Rhodopsins are seven-transmembrane proteins that contain retinal as a light-absorbing chromophore and a light-induced trans–cis isomerization of retinal triggers their activities. There are, however, 9 genomes from a high salinity environment, 8 were from the same site and showed little genetic variation. Phylogenetic analysis of the amino acid sequences of the rhodopsins encoded by the 56 identified genes revealed that the proteins belonged to four known rhodopsin clades: XLR (3 genes), NaR (1 gene), XeR (15 genes), and CyHR (24 genes) and one novel clade (13 genes); the novel rhodopsin clade consisted entirely of rhodopsin genes from cyanobacterial genomes so we named the clade “cyanorhodopsin” (CyR). All of the CyRs included Lys204N2098R in the seventh helix (helix G), which is known to make a Schiff base linkage between the rhodopsin protein moiety and the retinal chromophore in other rhodopsins. Heterologous rhodopsin gene expression analysis showed that the rhodopsins in the CyR clade function as light-driven outward H+ pumps.

The crystal structures of cell-free-synthesized N2098R and N4075R were determined at 2.65 Å and 1.9 Å resolution, respectively. The N2098R protein crystallized into space group C2221, with a N2098R trimer per asymmetric unit. The N2098R monomer is composed of seven transmembrane helices (helices A–G) and a long C-terminal helix. The long C-terminal helix is bent at the end of helix G, Gly215N2098R, and covers the cytoplasmic surface of helix C–F. A pentagonal cluster consisting of three water molecules adjacent to the Schiff base of Lys204, Asp74, and Asp200 plays an important role in proton transport (broken lines). In addition, the location of the putative proton release group comprising Glu182 and Glu192 (corresponding to Glu194BR and Glu204BR in BR) is also very similar. The overall structure of N2098R is similar to that of GR (RMSD 1.91 Å) and ASR (RMSD 1.40 Å), but the structural position of the water molecules and amino acids around the retinal and the putative exit region of the proton are quite different. To examine the amino acid residues crucial for the proton-transport activity of N2098R, mutants at the putative proton acceptor Asp74N2098R, proton donor Glu85N2098R, or counterion Asp200N2098R were examined. Replacement of these amino acids prevented light-mediated change of the pH of the cell suspensions despite expressed as well as wild type in E. coli cells, indicating that these residues are essential for proton transport; this finding provides further evidence that N2098R functions as a light-driven outward proton pump. A structural comparison revealed a high conformational similarity between N2098R and BR, and a mutant analysis confirmed that the putative proton donor and acceptor in N2098R both worked as expected.

>GSSGSSGMTQFWLWVGFIGMVIGCIYFGMKASAMRRREGMEFPLESFFITLWAAALYLTMILGETVTPINGQTVFWGRYIDWVVTTPLLLMELGVIAGLRPKLIAGVMGADIFMIVTGFIGAVEAPPYNYLWWLISTGSFLAILGSLLTEYSASAKRRNGRINSLFQTLRNILIVLWICYPIVWILGAEGFHVISVGWETLCYSVLDVCAKVGFGFVVVSAGNETLAQASNSDRIMETVHSYMQSEEREQSPYR[3x]> GAMDPGEETINSTQNKTRTKTTRPK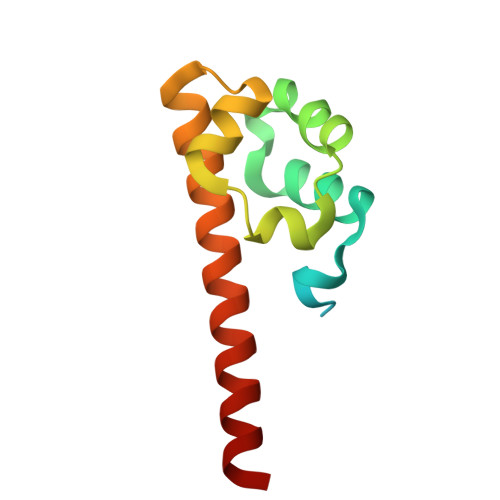AVYLWTVSDVLKWYRRHCGEYTQYEQLFAQHDITGRALLRITDSSLQRMGVTDNRDREAIWREIVKQRLKTDIMEIRDMERLNIY>[4x]MDIKINDITLGNNSPFVLFGGINVLESLDSTLQTCAHYVEVTRKLGIPYIFKASFDKANRSSIHSYRGVGLEEGLKIFEKVKAEFGIPVITDVHEPHQCQPVAEVCDVIQLPAFLAKQTDLVVAMAKTGNVVNI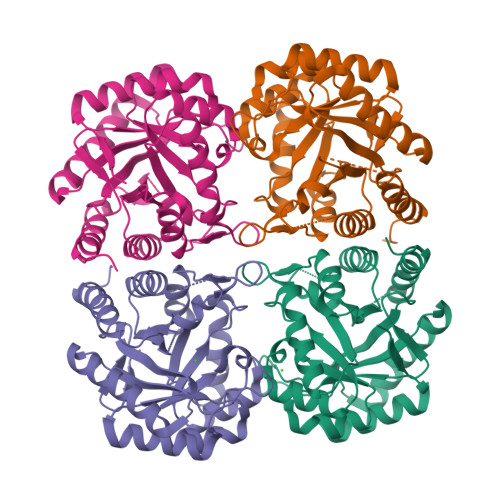KKPQFLSPSQMKNIVEKFHEAGNGKLILCERGSSFGYDNLVVDMLGFGVMKQTCGNLPVIFDVTHSLQTRDAGSAASGGRRAQALDLALAGMATRLAGLFLESHPDPKLAKCDGPSALPLHLLEDFLIRIKALDDLIKSQPILTIE> IVGGSNAKEGAWPWVVGLYYGGRLLCGASLVSSDWLVSAAACVYGRNLEPSKWTAILGLHMKSNLTSPQTVPRLIDEIVINPHYNRRRKDNAIAMMHLEFKVNYTDYI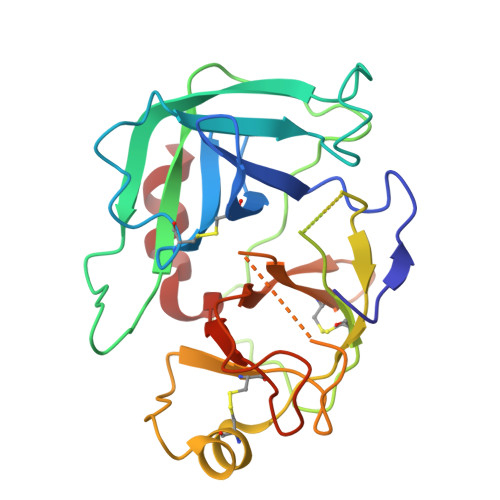QPICLPEENQVFPPGRNCSIAGWGTVVYQGTTANILQEADVPLLSNERCQQQMPEYNITENMICAGYEEGGIDSCQGDAGGPLMCQENNRWFLAGVTSFGYKCALPNRPGVYARVSRFTEWIQSFLH PsEst3, a psychrophilic esterase obtained from Paenibacillus sp. R4, which was isolated from the permafrost of Alaska, exhibits relatively high activity at low temperatures. Here, crystal structures of PsEst3 complexed with various ligands were generated and studied at atomic resolution, and biochemical studies were performed to analyze the structure–function relationship of PsEst3. The residues located in the active site, including the catalytic triad (Ser128, Asp199 and His227), were strictly conserved.

Four structures were obtained: a sulfate-bound form, the wild type bound to PMSF, a malonate-bound form of the S128A mutant and an apo form of the S128A mutant. Two unintentionally complexed ligands that were derived from the crystallization solution were detected in the PsEst3 structures: a sulfate and a malonate. Structural superposition of the sulfate-bound structure and the malonate-bound structure of the S128A mutant with the apo structure of the S128A mutant revealed r.m.s.d.s of 0.4 and 0.3 Å, respectively, indicating that the overall conformational changes caused by the ligands were not critical. In the sulfate-bound structure, a sulfate molecule occupied the active site near Ser128, interacting with Phe43, Arg44, Ser128 and His227 [Figs. 5(a) and 5(b)]. Compared with diethyl phosphonate, which mimicked the transition state interacting with the oxyanion hole, sulfate exhibited an approximate shift of 2.6 Å caused by hydrogen bonds between an O atom of sulfate and the N atoms of the 43-FR-44 main chain. Another O atom of sulfate was located near the oxyanion hole comprising the backbone N atoms of Arg129 and Phe43; however, its orientation did not directly mimic that of diethyl phosphonate.

> MGNAVVVKKDFRIDLENELFIRGEVTLVEDQIKKPVLVISHGFRGYKDWGFWPYVAAWFAERGFYVVHFDFSRVGALNSGADEASVQKLSTVSRELSDLDAILSNLREHRLPLAEQAETERISLLGHSRAGGSNIIFAAEHSYIGSVIAWNGGPPPKAAAGNPNPFINDDVEHNKQRFDTARLLASLTAPVLIIQGGKDREALLEGQQLLKEAAPNQTYISIPDADHSFGGEHPFHHTTPYLEEALEVTHSFITKHYLEHHHHHH>HHHHHHSSGLVPRGSHMASMSSNLSHKAYMIGAGIGNLSAAVYLIRDGEWNGEDITIMGLDMHGANDGESAATFQHQYGHRELGNDAGFINRGGRMLNEETYENLWDVLSAVPSLDNPGKSVTDDILDFDHAHPTHDVARLIDRDGIRNKGENDYKHMQFDNKDRYLLTKLMTMPESDEAKLDDISIEQWFEETPHFFTTNFWYMWETTFAFKRVSSAMELRRYMNRMILEFSR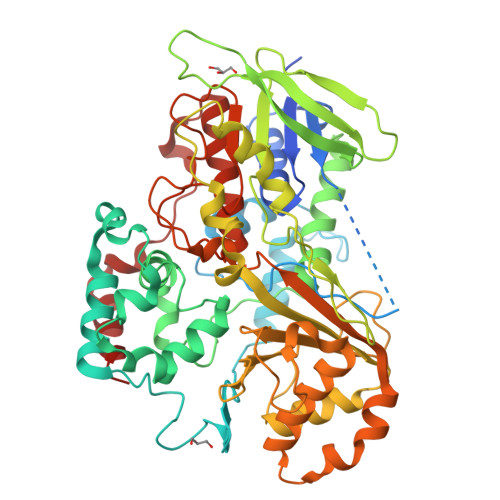IQTLAGVTRSPYNQYESIILPMRTFLEGKGVKFVNELKITEFVFKDTPLRDEIIVTGLDYENVRTGEKGRIDVAEGDFVFDTNGSITDSSSIGDLDTPIVEDMRYAPSALLWKQATEHFYDLGNPDKFFGDRAQSEWTSFTVTTSSHELINEISRITKQLPGNALNTFVDSNVLLSIVVHHQPHYHAQKENEGVFWGYCLFPRKDGDYVKKPFIEMTGREMLEETLGHLEALDESGTLAARRQEIMDSVVNSIPSHMPYASALFNRRAVGDRPLVVPKHSKNLAFISQFAELPFDMVFTEQYSVRCAQVAVYKFLGIPEDKLTKMHHYEKDPKVLAKAAVTMFR[2x]>SRAPYSGPQDLAALLEQIGCLKYLQVFEEQDVDLREFLTLTESDLKEIGITLFGPKRKMT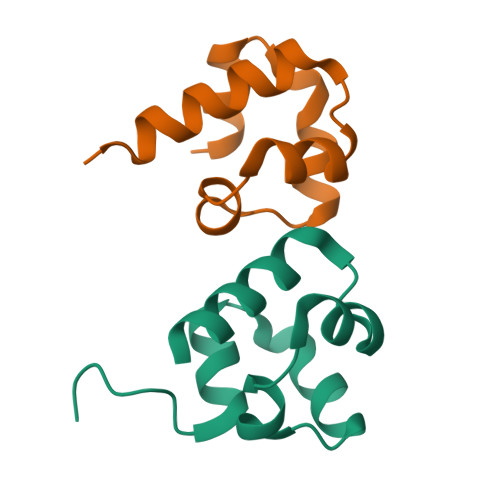SAIARWHSSAR[2x];>[2x]STITDEDELTGILKKLSLEKYQPIFEEQEVDMEAFLTLTDGDLKELGIKTDGSRQQILAAISELNAGKGRE>[3x]MLSETELRALKKLSTTTSRVVGDSTLALPSNVKLSKGEVEKIAVTKKEMFDELAQCNLPTIELITREHTFNGDVIRFAAWLFLMNGQKLMIANNVAVRMGMQYATNLAGNNVKITYVTSNNVVKLGHIAAGVLANPYSNKGSGLFITYEHN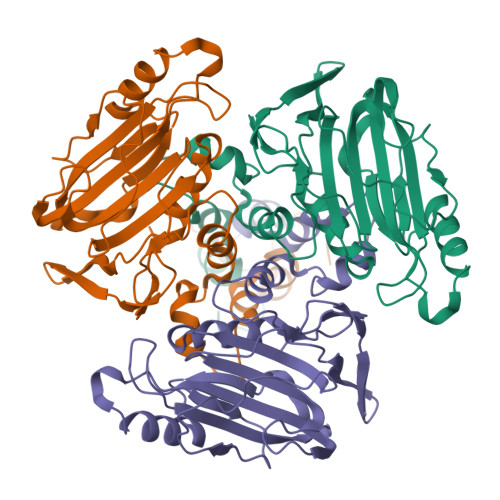LISNQIETGKVCVLFITSLSTTASSTNSFAYSACSVPIEDWDFNMIKLTAETSCASLTAMTNLVNSLVPGERTRPVGLYVDIPGVTVTTSASSGSLPLTTIPAVTPLIFSAYTKQVEEVGVINTLYALSYLP>MSYRIVVDPKKVVKPISRHIYGHFTEHLGRCIYGGIYEEGSPLSDERGFRKDVLEAVKRIKVPNLRWPGGNFVSNYHWEDGIGPKDQRPVRFDLAWQQEETNRFGTDEFIEYCREIGAEPYISINMGTGTLDEALHWLEYCNGKGNTYYAQLRRKYGHPEPYNVKFWGIGNEMYGEWQVGHMTADEYARAAKEYTKWMKVFDPTIKAIAVGCDDPIWNLRVLQEAGDVIDFISYHFYTGSEDYYETVSTVYLLKERLIGVKKLIDMVDTARKRGVKIALDEWNVWYRVSDNKLEEPYDLKDG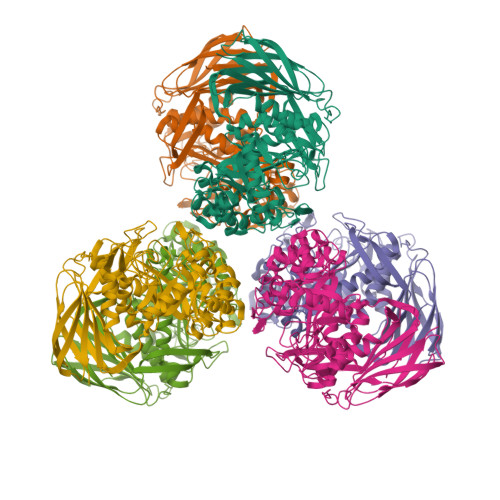IFACGVLVLLQKMSDIVPLANLAQLVNALGAIHTEKDGLILTPVYKAFELIVNHSGEKLVKTHVESETYNIEGVMFINKMPFSVENAPFLDAAASISEDGKKLFIAVVNYRKEDALKVPIRVEGLGQKKATVYTLTGPDVNARNTMENPNVVDITSETITVDTEFEHTFKPFSCSVIEVELE[12x]> MTMVLPGVSYNETLLTQASNDDPVTMPLFIGYTPPDTAIPVTVMQPVSVGSLTQANSLFGQRGTLAYSLRHFFENGGLQCYVLPLGPGKGEPAARLQELIAALQTPQMLETLLADDKTGLVLVPELSELNEVSSTSLSAEGVDAAEVDADALWYQGWQVLLTLCRQAPQRFALLELPEDPASAVTLTQQSFSADQCQRGAAWWPRLETSYQDESSAPVVLSPLPAVAAAIQRSAHDNGVWKAPANIALAKTRRPTQSILTSQALLDNQGVSCNLIRSFVGKGVRLWGCRTLLNEENTAWRYIQIRLLVSSVEHYLSKLARAYLFEPNTAPTWMKLKGQVWTWLRQQWLAGAFFGTVEDEAFSLSIGLDETMTEDDIRHGKMILQVRLALLAPAEFIAISLTLDLRDG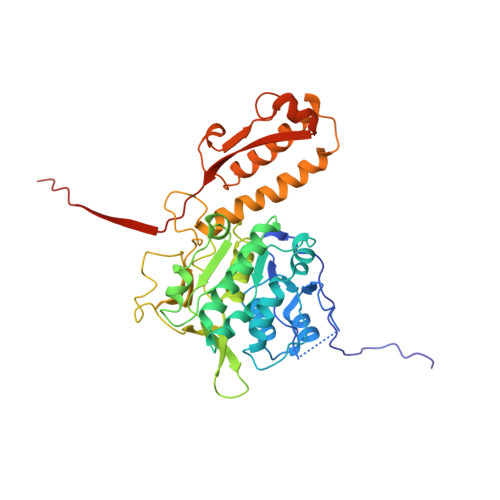TASAQTGGQS>[2x]GPNPYDRKRQDKAPVGLKNVGNTCWFSAVIQSLFNLLEFRRLVLNYKPPSNAQDLPRNQKEHRNLPFMRELRYLFALLVGTKRKYVDPSRAVEILKDAFKSNDSQQQDVSEFTHKLLDWLEDAFQMKAEEETDEEKPKNPMVELFYGRFLAVGVLEGKKFENTEMFGQYPLQVNGFKDLHECLEAAMIEGEIESLHSENSGKSGQEHWFTELPPVLTFELSRFEFNQALGRPEKIHNKLEFPQVLYLDRYMHRNREITRIKREEIKRLKDYLTVLQQRLERYLSYGSGPKRFPLVDVLQYALEFASSKPVCTSPVDDIDASSPPSGSIPSQTLPSTTEQQGALSSELPSTSPSSVAAISSRSVIHKPFTQSRIPPDLPMHPAPRHITEEELSVLESCLHRWRTEIENDTRDLQESISRIHRTIELMYSDKSMIQVPYRLHAVLVHEGQANAGHYWAYIFDHRESRWMKYNDIAVTKSSWEELVRDSFGGYRNASAYCLMYINDKAQFLIQEEFNKETGQPLVGIETLPPDLRDFVEEDNQRFEKELEEWDAQLAQKALQE

The evolutionarily related deubiquitinating enzymes (DUBs) USP25 and USP28 comprise an identical overall domain architecture but are functionally non-redundant: USP28 stabilizes c-MYC and other nuclear proteins, and USP25 regulates inflammatory TRAF signaling. USP25 and USP28 share an identical domain structure and highly homologous catalytic domains. USP catalytic domains are usually around 350 amino acids (aa) in length; however, in USP25/28, the catalytic domains span ∼550 aa due to a large, conserved insertion of unknown function at a common insertion point between USP boxes 4 and 5 (Ye et al., 2009). Active enzymes form distinctively shaped dimers, with a dimerizing insertion spatially separating independently active catalytic domains.

Attempts to crystallize this intriguing USP25 tetramer eventually resulted in a 2.9-Å crystal structure. Interestingly, USP25 formed a dimer of dimers, wherein the distinctive, V-shaped dimerization interface of one dimer inserted between catalytic domains of a second dimer, forming a symmetric tetramer. Tetramerization orients catalytic domains such that ubiquitin-binding sites face outward and are accessible to solvent. Blocking loops 1 and 2, regulatory elements that line the C terminus of a bound ubiquitin (Clerici et al., 2014), are pried open by direct interactions with the insertion stalk provided by the second dimer. Importantly, we found that the tetramer was autoinhibited. A 14-residue section of the linker that is disordered in USP28 becomes ordered in USP25 and binds the ubiquitin binding site in a neighboring catalytic domain in the tetramer; this way all four catalytic domains are unable to bind ubiquitin. The AIM spans across the ubiquitin-binding site at the connection between the Palm and Fingers subdomains. Importantly, strong anchoring is provided by a section of the AIM, aa 519–524, that inserts itself into the core of the catalytic domain, occupying an unexpected pocket below the α5 helix. In particular, Pro521 and Phe522 rest deeply within the USP core, and this interaction acts as a wedge that pushes the α5 helix away from the catalytic domain, e.g., when compared to apo and Ub-PA-bound states of USP28. We conclude that USP25 forms an autoinhibited dimer of dimers, in which the insertion not only performs the key underlying dimerization role but also acts, via its AIM, as a regulatory element.> MKPPQFTWAQWFETQHINMTSQQCTNAMQVINNYQRRCKNQNTFLLTTFANVVNVCGNPNMTCPSNKTRKNCHHSGSQVPLIHCNLTTPSPQNI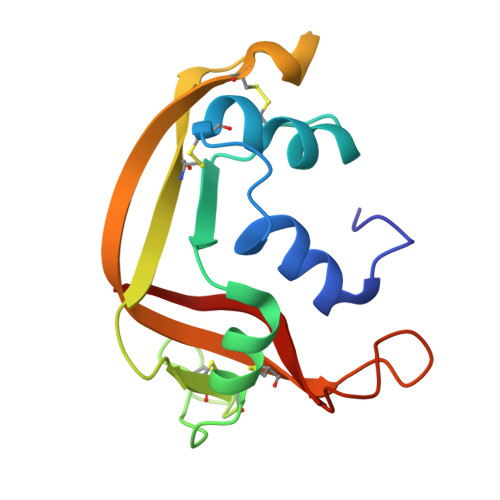SNCRYAQTPANMFYIVACDNRDQRRDPPQYPVVPVHLDRII>GSMSTRESFNPESYELDKSFRLTRFTELKGTGCKVPQDVLQKLLESLQENHFQEDEQFLGAVMPRLGIGMDTCVIPLRHGGLSLVQTTDYIYPIVDDPYMMGRIACANVLSDLYAMGVTECDNMLMLLGVSNKMTDRERDKVMPLIIQGFKDAAEEAGTSVTGGQTVLNPWIVLGGVATTVCQPNEFIMPDNAVPGDVLVLTKPLGTQVAVAVHQWLDIPEKWNKIKLVVTQEDVELAYQEAMMNMARLNRTAAGLMHTFNAHAATDITG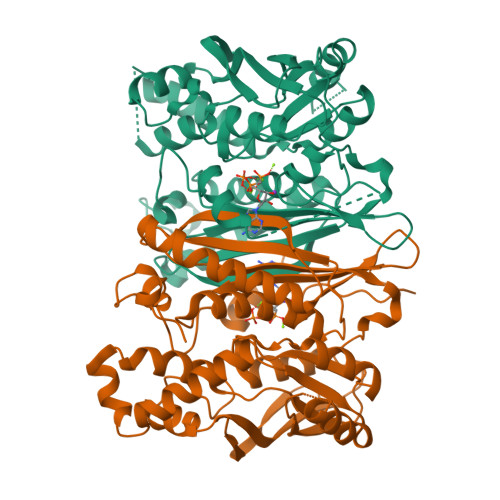FGILGHAQNLAKQQRNEVSFVIHNLPVLAKMAAVSKACGNMFGLMHGTCPETSGGLLICLPREQAARFCAEIKSPKYGEGHQAWIIGIVEKGNRTARIIDKPRIIEVAPQVATQNVNPTPGATS[2x]> MLTPTPDSSPRSTSSPSQSKNGSFTPRTANILKPLMSPPSREE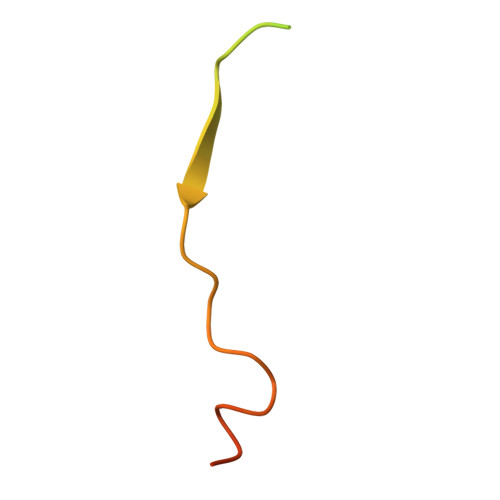IMATLLDHD>MVLYFIGLGLYDERDITVKGLEIAKKCDYVFAEFYTSLMAGTTLGRIQKLIGKEIRVLSREDVELNFENIVLPLAKENDVAFLTPGDPLVATTHAELRIRAKRAGVESYVIHAPSIYS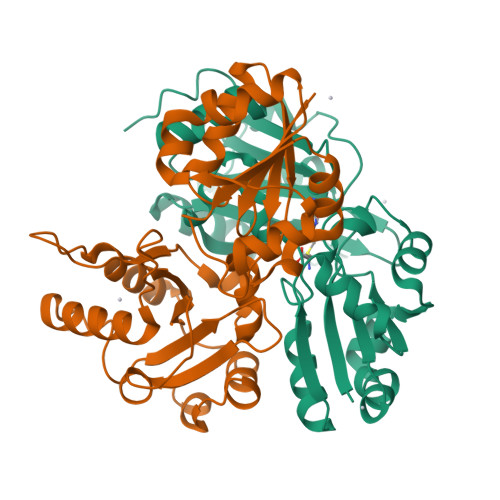AVGITGLHIYKFGKSATVAYPEGNWFPTSYYDVIKENAERGLHTLLFLDIKAEKRMYMTANEAMELLLKVEDMKKGGVFTDDTLVVVLARAGSLNPTIRAGMVKDLIREDFGDPPHILIVPGKLHIVEAEYLVEIAGAPREILRVNV[2x]> MTENILRKSDEEIQKEITARVKALESMLIEQGILTTSMIDRMAEIYENEVGPHLGAKVVVKAWTDPEFKKRLLADGTEACKELGIGGLQGEDMMWVENTDEV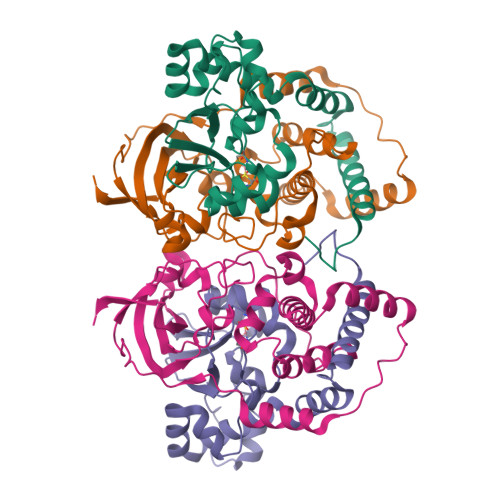HHVVVCTLCSCYPWPVLGLPPNWFKEPQYRSRVVREPRQLLKEEFGFEVPPSKEIKVWDSSSEMRFVVLPQRPAGTDGWSEEELATLVTRESMIGVEPAKAV;> MNGVYDVGGTDGLGPINRPADEPVFRAEWEKVAFAMFPATFRAGFMGLDEFRFGIEQMNPAEYLESPYYWHWIRTYIHHGVRTGKIDLEELERRTQYYRENPDAPLPEHEQKPELIEFVNQAVYGGLPASREVDRPPKFKEGDVVRFSTASPKGHARRARYVRGKTGTVVKHHGAYIYPDTAGNGLGECPEHLYTVRFTAQELWGPEGDPNSSVYYDCWEPYIELVDT> GAMGSMATYEVLCEVARKLGTDDREVVLFLLNV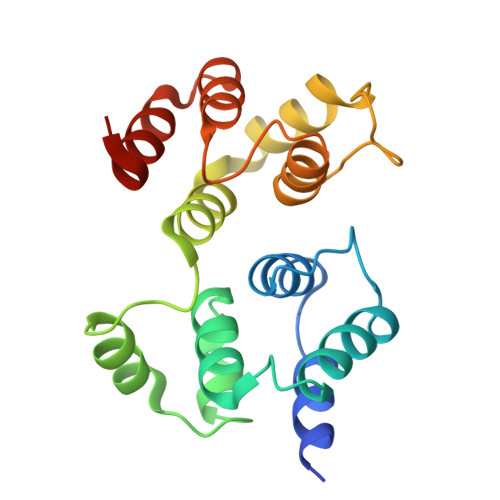FIPQPTLAQLIGALRALKEEGRLTFPLLAECLFRAGRRDLLRDLLHLDPRFLERHLAGTMSYFSPYQLTVLHVDGELCARDIRSLIFLSKDTIGSRSTPQTFLHWVYCMENLDLLGPTDVDALMSMLRSLSRVDLQRQVQTLMGLHLSGP> GSMQNTTHDNVILELTVRN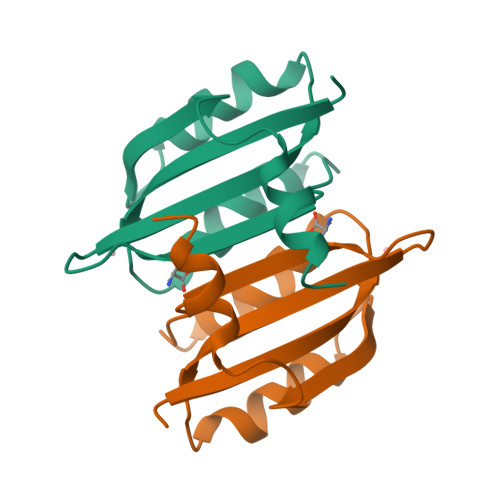HPGVMTHVCGLFARRAFNVEGILCLPIQDSDKSHIWLLVNDDQRLEQMISQIDKLEDVVKVQRNQSDPTMFNKIAVFFQ> GVPTCLLPGSNQFLTTDDHSSAPAFPDFSPTPEMHIPGQVHSMLEIVQIESMMEINNVNDASGVERLRVQISAQSDMDQL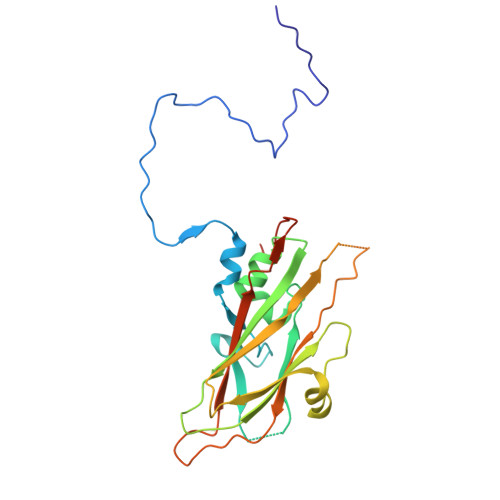LFNIPLDIQLEGPLRNTLLGNISRYYTHWSGSLEMTFMFCGSFMTTGKLIICYTPPGGSSPTDRMQAMLATHVVWDFGLQSSITIIIPWISGSHYRMFNTDAKAINANVGYVTCFMQTNLVAPVGAADQCYIVGMVAAKKDFNLRLMRDSPDIGQSAILPEQ>[2x]GSSGSSGMAPWRKADKERHGVAIYNFQGSGAPQLSLQIGDVVRIQETCGDWYRGYLIKHKMLQGIFPKSFIHIKEVTVEKRRNTENIIP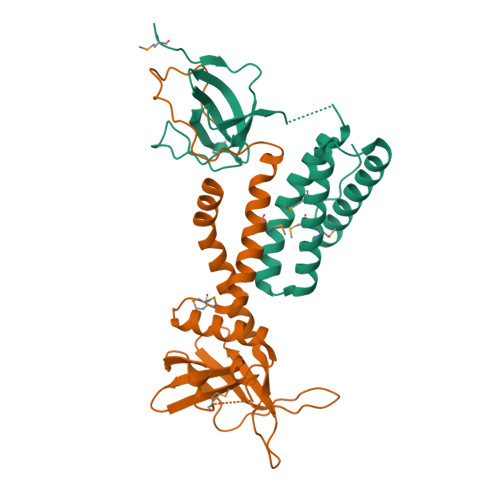AEIPLAQEVTTTLWEWGSIWKQLYVASKKERFLQVQSMMYDLMEWRSQLLSGTLPKDELKELKQKVTSKIDYGNKILELDLIVRDEDGNILDPDN;>[2x]GSSGSSGPILELKEKIQPEILELIKQQRLNRLVEGTCFRKLNARRRQDKFWYCRLSPNHKVLHYGDLEESPQGEVPHDSLQDKLPVADIKAVVTGKDCPHMKEKGALKQNKEVLELAFSILYDSNCQLNFIAPDKHEYCIWTDGLNALLGKDMMSDLTRNDLDTLLSMEIKLRLLDLENIQIPDAPPPIPKEPSNYDFVYDCN> SNAMSSSSSPPHQLNHFSDVANKAANAAGDVIRKYFRKNNFDIIHKNDLSPVTIADQSAEE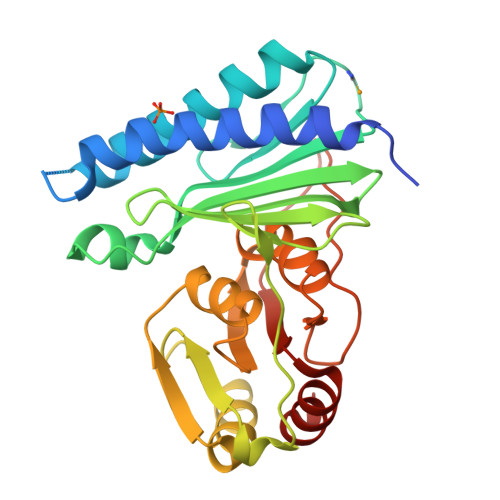AMVSVILDNFPSHAVYGEEKGWRCKQDSADYVWVLDPIDGTKSFITGKPLFGTLIALLQNGTPILGIIDQPVLKERWIGITGKRTTLNGQEVSTRTCADLSQAYLYTTSPHLFSGDAEEAFIRVRDKVKIPLYGCDCYAYALLSSGFVDLVVESGLKPYDFLALIPVIEGSGGVITDWKGHQLRWEASPLSIATSFNVVAAGDKQIHQQALDSLQW(3R)-3-azanyl-4-(4-chlorophenyl)-1-[(3S,4R)-3-(4-chlorophenyl)-4-(hydroxymethyl)pyrrolidin-1-yl]butan-1-one | C21 H24 Cl2 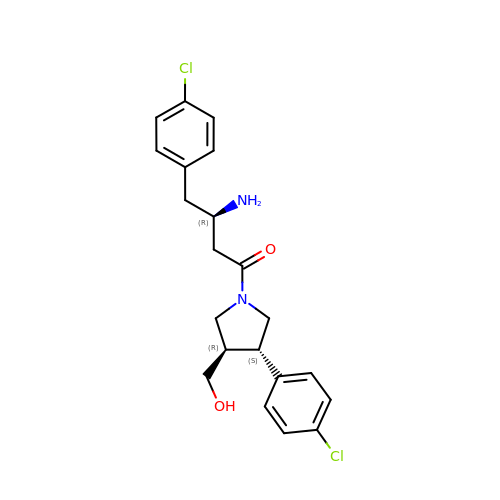N2 O2 | ZFSKJGRASNTEBX-NSISKUIASA-N The baseplate is a complex structure at the tip of bacteriophage tails that serves multiple roles, including host recognition and binding, cell wall penetration, and ejection of the phage DNA. We have determined the structure of the baseplate from bacteriophage 80α, a representative of phages involved in host pathogenicity and in the mobilization of MGEs in S. aureus. Phage 80α is a typical staphylococcal siphovirus with a 43.8 kbp genome and a 63 nm icosahedral capsid, attached to a 190 nm long flexuous tail that is capped by an ornate baseplate. Here, we have determined the cryo-EM structure of the 80α baseplate at 3.75 Å resolution, allowing most of the baseplate proteins and part of the tail to be modeled in atomic detail.

Atomic models for MTP (gp53), Dit (gp58), RBP (gp61), and parts of Tal (gp59), FibL (gp62), FibU (gp68) and TMP (gp57) were built into either the C6 or C3 baseplate reconstructions, using I-TASSER models as starting points, complemented with real-space refinement in PHENIX. In total, 72 polypeptides comprising 7 different proteins were included in the final model. The baseplate is 298 Å wide and 271 Å tall and consists of six peripheral structures surrounding a core that represents a continuation of the tail. In a complete tail ring, one of these β-sheets forms a 24-stranded, highly negatively charged β-barrel—42 Å in diameter—lining the tail lumen, presumably providing a slippery tube for the DNA during infection. The Dit hexamer constitutes the hub of the baseplate, forming an adaptor between the sixfold symmetric tail and the threefold symmetric Tal protein, as well as the attachment point for the six RBP trimers. The Tal NTD (residues 1–331) consists of two tail tube domains (TT1 and TT2) that form a quasi-sixfold adapter to the Dit hexamer. In the Tal trimer, these helices form a twisted tripod that occludes the opening of the lumen. After accounting for the plug and rod helices, there were three additional, well-ordered α-helical densities forming a second tripod interlaced with that of the Tal plug. This density matched the C-terminal residues 1135–1154 of TMP. RBP is a trimeric protein consisting of four domains: an N-terminal α-helical coiled-coil “stem” domain (residues 1–142) that is folded by 155° at a central hinge; a five-bladed β-propeller “platform” domain (residues 143–442) that was previously suggested to bind to the GlcNAc residues of WTA on the host cell surface; and two highly similar C-terminal “tower” domains (residues 443–636), each consisting of a bent β-sheet superposed by an α-helix. Six such trimers surround the baseplate core, making up the bulk of the observed peripheral structures.

>MANMKNSNDRIILFRKAGEKVDATKMLFLTEYGLSHEADTDTEDTMDGSYNTGGSVESTMSGTAKMFYGDDFADEIEDAVVDRVLYEAWEVESRIPGKNGDSAKFKAKYFQGFHNKFELKAEANGIDEYEYEYGVNGRFQRGFATLPEAVTKKLKATGYRFHDTTKEDALTSEDLTAIPQPKVDSSTVTPGEV[12x];>[6x]MDIELTKKDGTVIKLSEYGFIVNDIVIDSMQINTKYQDKENMNGRILMGSNYISRDIVVPCFCKVKNRSDIAYMRDMLYSLTTDIEPMYLREIRRKEELNYRFTQPTSDDYVKLDKNNFPDYEYSRHDQQIYVNGKQYKVIFNGVINPKQKGNKVSFELKFETTELPYGESIGTSLELEENKKVGLWSFDFNIDWHAGGDKRKYTFENLSKGTVYYHGSAPNDQFNMYKKITIILGEDTESFVWNLTHAEIMKIEGIKLKAGDRIVYDSFRVYKNGVEISTETNISQPKFKYGANKFEFNQTVQKVQFDLKFYYK;>[3x]MTITIKPPKGNGAPVPVETTLVKKVNADGVLTFDILENKYTYEVINAIGKRWIVSHVEGENDKKEYVITVIDRKSEGDRQLVECTAREIPIDKLMIDRIYVNVTGSFTVERYFNIVFQGTGMLFEVEGKVKSSKFENGGEGDTRLEMFKKGLEHFGLEYKITYDKKKDRYKFVLTPFANQKASYFISDEVNANAIKLEEDASDFATFIRGYGNYSGEETFEHAGLVMEARSALAEIYGDIHAEPFKDGKVTDQETMDKELQSRLKKSLKQSLSLDFLVLRESYPEADPQPGDIVQIKSTKLGLNDLVRIVQVKTIRGINNVIVKQDVTLGEFNREQRYMKKVNTAANYVSGLNDVNLSNPSKAAENLKSKVASIAKSTLDLMSRTDLIEDKQQKVSSKTVTTSDGTIVHDFIDKSNIKDVKTIGTIGDSVARGSHAKTNFTEMLGKKLKAKTTNLARGGATMATVPIGKEAVENSIYRQAEQIRGDLIILQGTDDDWLHGYWAGVPIGTDKTDTKTFYGAFCSAIEVIRKNNPASKILVMTATRQCPMSGTMIRRKDTDKNKLGLTLEDYVNAQILACSELDVPVYDAYHTDYFKPYNPAFRKSSMPDGLHPNERGHEVIMYELIKNYYQFYG;>[3x]MTEYKIKATIEASVAKFKRQIDSAVKSVQRFKRVADQTKDVELNANDKKLQKTIKVAKKSLDAFSNKNVKAKLDASIQDLQQKILESNFELDKLNSKEASPEVKLQKQKLTKDIAEAENKLSELEKKRVNIDVNADNSKFNRVLKVSKASLEALNRSKAKAILDVDNSVANSKIKRTKEELKSIPNKTRSRLDVDTRLSIPTIYAFKKSLDALPNKKTTKVDVDTNGLKKVYAYIIKANDNFQRQMGNLANMFRVFGTVGSNMVGGLLTSSFSILIPVIASVVPVVFALLNAIKVLTGGVLALGGAVAIAGAGFVAFGAMAISAIKMLNDGTLQASSATNEYKKALDGVKSAWTDIIKQNQSAIFTTLANGLNTVKTAMQSLQPFFSGISRGMEEASQSVLKWAENSSVASRFFNMMNTTGVSVFNKLLSAAGGFGDGLVNVFTQLAPLFQWSADWLDRLGQSFSNWANSAAGENSITRFIEYTKTNLPIIGNIFKNVFAGINNLMNAFSGSSTGIFQSLEQMTAKFREWSEQVGQSQGFKDFVSYIQTNGPLIMQLIGNIARGLVAFATAMAPIASAVLRVAVAITGWIANLFEAHPATAQLVGVIITLVGAFRFLIAPILAVMDFLGPLAARLVALVTKFGWAKTGTLVLSKAMTSLKGPIKLVTAIFQLLFGKIGLIRNAITGLVTVFGILGGPITIVIGVIAALIAIFVLLWNKNEGFRNFIINAWNAIKTFMVNVWNVLKAVASVVWNAILTAITTAVSNVYNFIMIVWNQIVAYLQGLWNGIIAIATTVWNLLVTIITTVFTTIMTIVMTIWTAIWTFLSTIWNTIITIATTIWNLLVTVITTVFTTIMTIAMTIWNAIWTFLQTLWNTIVTVATKVWNAITTAISTALQAAWSFISNIWNTIWSFLSGILTTIWNKVVSIFTQVVSTISDKMSQAWNFIVTKGMQWVSTITSTLINFVNRVIQGFVNVVNKVSQGMTNAVNKIKSFIGDFVSAGADMIRGLIRGIGQMAGQLVDAAKNVAKKALDAAKSALGIHSPSREFMDVGMYSMLGFVKGIDNHSSKVIRNVSNVADKVVDAFQPTLNAPDISSITGNLSNLGGNINAQVQHTHSIETSPNMKTVKVEFDVNNDALTSIVNGRNAKRNSEYYL;>[18x]MDNKLITDLSRVFDYRYVDENEYNFKLISDMLTDFNFSLEYHRNKEVFAHNGEQIKYEHLNVTSSVSDFLTYLNGRFSNMVLGHNGDGINEVKDARVDNTGYDHKTLQDRLYHDYSTLDAFTKKVEKAVDENYKEYRATEYRFEPKEQEPEFITDLSPYTNAVMQSFWVDPRTKIIYMTQARPGNHYMLSRLKPNGQFIDRLLVKNGGHGTHNAYRYIGNELWIYSAVLDANENNKFVRFQYRTGEITYGNEMQDVMPNIFNDRYTSAIYNPIENLMIFRREYKASERQLKNSLNFVEVRSADDIDKGIDKVLYQMDIPMEYTSDTQPMQGITYDAGILYWYTGDSKPANPNYLQGFDIKTKELLFKRRIDIGGVNNNFKGDFQEAEGLDMYYDLETGRKALLIGVTIGPGNNRHHSIYSIGQRGVNQFLKNIAPQVSMTDSGGRVKPLPIQNPAYLSDITEVGHYYIYTQDTQNALDFPLPKAFRDAGWFFDVLPGHYNGALRQVLTRNSTGRNMLKFERVIDIFNKKNNGAWNFCPQNAGYWEHIPKSITKLSDLKIVGLDFYITTEESNRFTDFPKDFKGIAGWILEVKSNTPGNTTQVLRRNNFPSAHQFLVRNFGTGGVGKWSLFEGKVVE;>MVVDNFSKDDNLIELQTTSQYNPVIDTNISFYESDRGTGVLNFAVTKNNRPLSISSEHVKTFIVLKTDDYNVDRGAYISDELTIVDAINGRLQYVIPNEFLKHSGKVHAQAFFTQNGSDNVVVERQFSFNIENDLVSGFDGITKLVYIKSIQDTIEAVGKDFNQLKQNMADTQTLIAKVNDSATKGIQQIEIKQNEAIQAITATQTSATQAVTAEFDKIVEKEQAIFERVNEVEQQINGADLVKGNSTTNWQKSKLTDDYGKAIESYEQSIDSVLSAVNTSRIIHITSATDAPSFKDIGTVDTPKEDGVDDGSDIPVAPNTLGKSGVLVVYVVDDSTARATWYPDDSNDEYTKYKISGTWYPFYKKNDGDLTKQFVEETSNNALNQAKQYVDDKFGTTSWQQHKMTEANGQSIQVNLNNAQGDLGYLTAGNYYATRVPDLPGSVESYEGYLSVFVKDDTNKLFNFTPYNSKKIYTRSITNGRLEQQWTVPNEHKSTVLFDGGANGVGTTINLTEPYTNYSILLVSGTYPGGVIEGFGLTALPNAIQLSKANVVDSDGNGGGIYECLLSKTSSTTLRIDNDVYFDLGKTSGSGANANKVTITKIMGWK[18x];>[12x]MYKIKDVETRIKNDGVDLGDIGCRFYTEDENTASIRIGINDKQGRIDLKAHGLTPRLHLFMEDGSIFKNEPLIIDDVVKGFITYKIPKKVIKHAGYVRCKLFLEKEEEKIHVANFSFNIVDSGIESAVAKEIDVKLVDDAITRILKDNATDLLSKDFKEKIDKDVISYIEKNESRFKGAKGDKGEPGQPGAKGEAGKKGEQGAPGKNGTVVSINPDTKMWQIDGKDTDIKAEPELLDKINIANVEGLEDKLQEVEKIKDTTLNDSKTYTDTKIAELVDSAPESMNTLRELAEAIQNNSISESVLQQIGSKVSTEDFEEFKQTLNDLYAPKNHNHDERYVLSSQAFTKQQADSLYQLKSASQPTVKIWTGTENEYNYIYQKDPNTLYLIKG>ACGLVASNLNLKPGECLRVRGEVAADA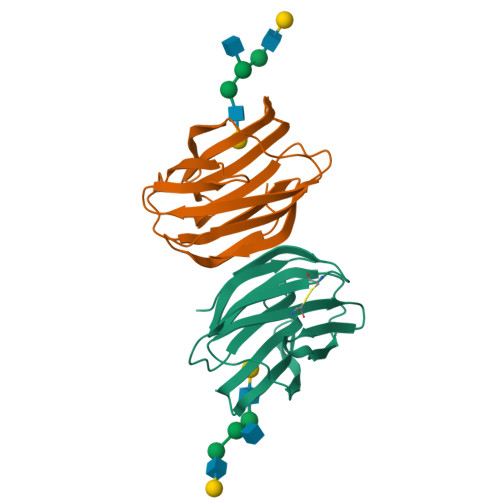KSFLLNLGKDDNNLCLHFNPRFNAHGDVNTIVCNSKDAGAWGAEQRESAFPFQPGSVVEVCISFNQTDLTIKLPDGYEFKFPNRLNLEAINYLSAGGDFKIKCVAFE[4x]> SNAMTTSAQSVLELLPAVDIVDGQAVRLLQGEAGSETSYGTPLEAALNWQNDGAEWVHMVDLDAAFGRGNNAALISDVVSQLNVKVELSGGLRDDESLERALELGVARVNLG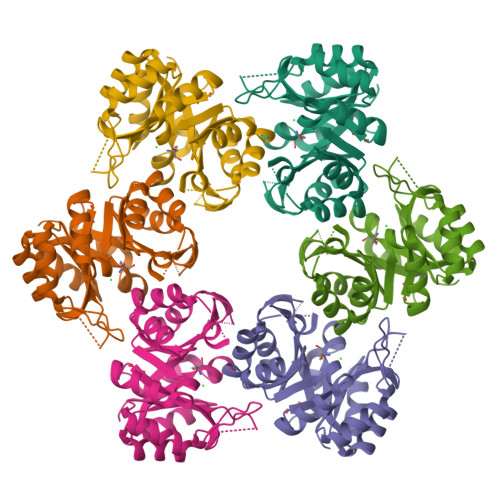TAALENPEWTRKAIDRFGDKIAVGLDVRGTTLAGRGWTKEGGDLWEVLARLEDAGCARYVVTDVTKDGTLQGPNVELLRQMVEKTGKPVVASGGISSLEDLRVLRELVPLGVEGAIVGKALYAGAFTLPEALDVAGRR> MGSGSGDDDDKLALSPESRLAAAWDALIAQPA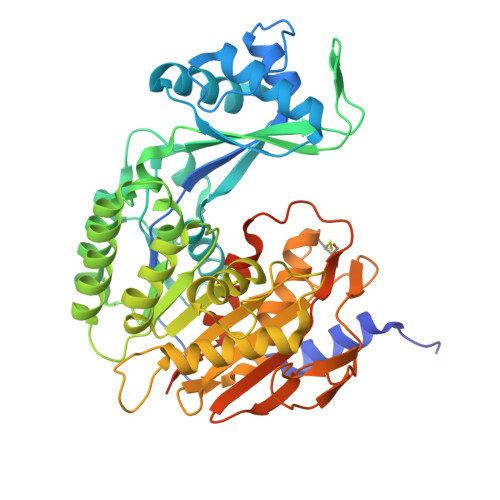RRWRRVAVGVNACVDVVISGVKLLQALGLSPGSGKDHAILHSRSDLEEAFLYFMGKGAAAERFFSDKETFHDIAQAASEFPGAQHYVGGNAALIGQRFAANTDLKVLLCGPIGPKLHELLDDNVFVPPESLQEEDEFHLILEYLAGEEWGPFKAPHANRFIFSHDLSNGAMNMLEVFVSSLEEFQPDLVVLSGLHMMEGQSKELQRKRLLEVVTAISDIPTGIPVHLELASMTNRELMSSIVHQVFPAVASLGLNEQELLFLSQSASGPHSSLSSWDGVPDVGMVSDILFWILKEHGRSENRSSDLTRIHFHTLVYHILATVDGHWANQLAAVAAGARVAGTQACATETIDTNRVSLRAPQEFTTSHLESGSRIVLNPDKPVVEWHREGITFHFTPVLVCKDPVRTVGLGDAISAEGLFYSEARPDKGQLQGKPIPNPLLGLDSTRTGHHHHHH>MLNRVVLVGRLTKDPELRSTPNGVNVGTFTLAVNRTFTNAQGEREADFINVVVFKKQAENVKNYLSKGSLAGVDGRLQTRNYENKDGQRVFVTEVVADSVQFLEPKNNNQ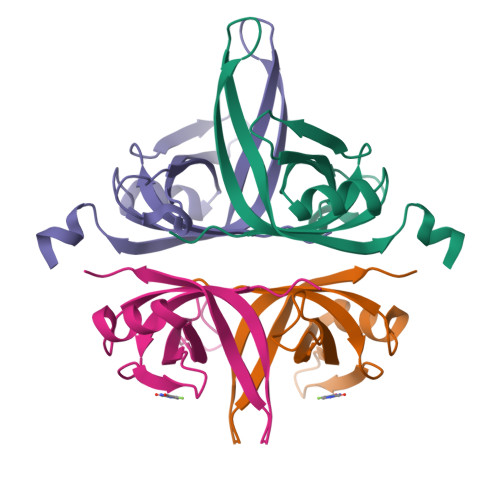QQHHHHHH[2x]> MRGSHHHHHHGRSRSLNPLSTPQFDSTDETPASYNLAVRRAAPAVVNVYNRGLNTNS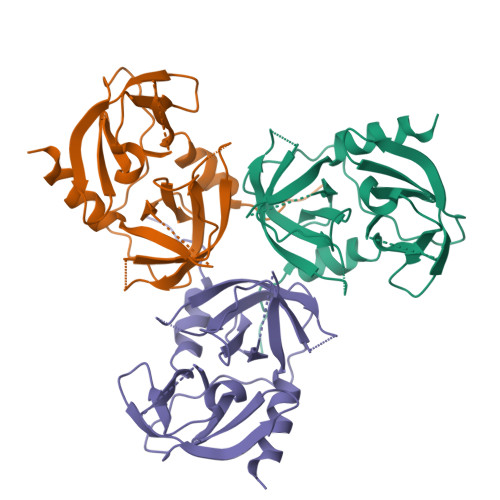HNQLEIRTLGSGVIMDQRGYIITNKHVINDADQIIVALQDGRVFEALLVGSDSLTDLAVLKINATGGLPTIPINARRVPHIGDVVLAIGNPYNLGQTITQGIISATGAIGLNPTGRQNFLQTDASINHGNSGGALVNSLGELMGINTLSFDKSNDGETPEGIGFAIPFQLATKIMDKLIRDGRVIR Here we report the neutron crystal structure of a PLP-dependent enzyme, aspartate aminotransferase (AAT), a fold-type I PLP-dependent enzyme that reversibly converts l-aspartate and α-ketoglutarate to oxaloacetate and l-glutamate via a ping−pong bi−bi mechanism. Pyridoxal 5′-phosphate (PLP), the biologically active cofactor derived from pyridoxine, is one of the most ubiquitous cofactors found in nature, catalyzing ~140 different types of biochemical transformations. Recombinant porcine cytosolic AAT fortuitously packs as a biological and crystallographic homodimer, with the two active sites having different activities toward the substrate analog α-methylaspartic acid. In AAT, the protonated pyridine nitrogen of the PLP (N1-PLP) enhances charge delocalization through resonance, permitting the subsequent transamination reaction.

To probe the structural changes that occur upon internal aldimine SB protonation, we obtained a low-pH X-ray structure of AAT in the absence of substrate, in which both chains are in the internal aldimine state. At pH 4.0, the internal aldimine shows geometric differences near the SB of PLP compared to the neutron structure at pH 7.5. When the geometries of the internal aldimines (chain B) from the pH 7.5 and pH 4.0 structures were compared, two major differences were evident. The torsion angle between the SB C = N bond and the pyridinium ring, and the O…O distance between the Y225 hydroxyl and O3′ of PLP are different. In the pH 4.0 structure, the SB is 22° above the pyridinium ring plane, compared to 46° in the internal aldimine at pH 7.5. Additionally, in the pH 4.0 structure the O…O distance between the Y225 hydroxyl and O3′ of PLP is 2.9 Å, compared with 2.6 Å in the internal aldimine state at pH 7.5. In the other monomer of the pH 4.0 structure (chain A, with restricted motion), the corresponding torsion angle and the (Y225)O…O(O3′) distance are 26° and 3.0 Å, respectively. Protonation of the SB nitrogen of the internal aldimine at low pH appears to introduce an H bond between O3′ and the SB by reducing the torsion angle between SB and the pyridinium ring. However, protonation of O3′ cannot be ruled out as H atoms were not observed in the low pH X-ray structure. Forced protonation alters the PLP alignment, suggesting that the microenvironment involving Y225 and the phenolic oxygen (O3′) of PLP influence the SB protonation and reactivity.

>[2x]GMAPPSVFAEVPQAQPVLVFKLIADFREDPDPRKVNLGVGAYRTDDCQPWVLPVVRKVEQRIANNSSLNHEYLPILGLAEFRTCASRLALGDDSPALQEKRVGGVQSLGGTGALRIGAEFLARWYNGTNNKDTPVYVSSPTWENHNGVFTTAGFKDIRSYRYWDTEKRGLDLQGFLSDLENAPEFSIFVLHACAHNPTGTDPTPEQWKQIASVMKRRFLFPFFDSAYQGFASGNLEKDAWAIRYFVSEGFELFCAQSFSKNFGLYNERVGNLTVVAKEPDSILRVLSQMQKIVRVTWSNPPAQGARIVARTLSDPELFHEWTGNVKTMADRILSMRSELRARLEALKTPGTWNHITDQIGMFSFTGLNPKQVEYLINQKHIYLLPSGRINMCGLTTKNLDYVATSIHEAVTKIQ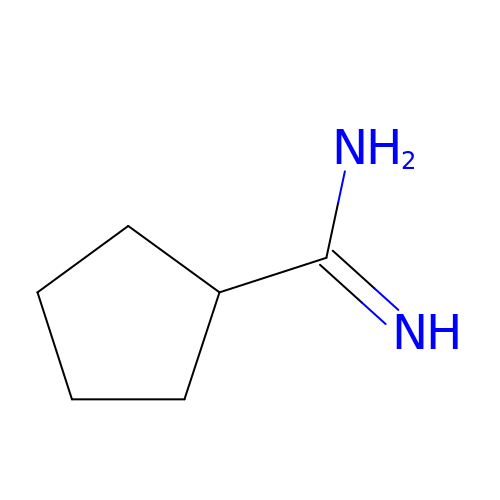cyclopentanecarboximidamide | C6 H12 N2 | RMALUJUDHRIMQN-UHFFFAOYSA-N>GSHMTITDVLKNTFNISPKPPRKFIAIDLGTTNSIAYIGGRGIIYNEASVMAYETGTKKLVALGEDARKLIGKTHDKIEIYTPLRNGAITDLRIAEEFIQHIGNRAKVQDVWKGSIVLIACPKSVTELERRAMVEMCKHLGADLVQVEEDTLMAALGAGANIFAPKGTFILDIGGGKTSAGIISAGGIVVSKSIKIAGNYIDEEILKYIRAKHTISIGVVTAEQIKKQIGSLYKGKETKKMVIFGRDVVTGMPKETEILDSEIRKLLISIFSSITQLVTDILESTPAELAGDAVMNGLLVSGGCAQISGLKEFLESYFQIPVKIAKNPQTAVIDGCIAYEKEIRDRLIEENKKNK[2x]

MreB is a bacterial protein belonging to the actin superfamily. This protein polymerizes into an antiparallel double-stranded filament that determines cell shape by maintaining cell wall synthesis. Here, we studied MreB3 and MreB5 in Spiroplasma eriocheiris (SpeMreB3 and SpeMreB5, respectively), a model organism for studying Spiroplasma swimming. SpeMreB3 adopts a canonical actin fold composed of four subdomains (IA, IB, IIA and IIB) and consists of the same secondary structure elements as CcMreB, Thermotoga maritima (Tm) MreB and SciMreB5, except for the C-terminal region.

The crystal structures of nucleotide-free (Nf) SpeMreB3 and its AMPPNP complex were determined at 1.90 and 1.75 Å resolution. The SpeMreB3-AMPPNP complex crystal includes two molecules (Mol-A and Mol-B) with an RMSD value estimated for Cα atoms of 0.891 Å. Thus, the SpeMreB3-AMPPNP complex crystal also contains antiparallel pairs of the protofilaments, although their arrangement differs from that of the Nf-SpeMreB3 crystal. The angle composed of centroids of subdomains IIB-IIA-IA (ω2) was more constant than ω1 among our crystal structures (ω2 = 88.9° for SpeMreB3-AMPPNP complex Mol-A, 90.3° for Mol-B and 91.2° for Nf-SpeMreB3), indicating that major structural changes upon nucleotide binding contribute to swing the subdomain IB. These conformational changes lead to the interaction between subdomains IIA and IB', which are absent in the Nf-SpeMreB3 protofilament. The interaction in SpeMreB3-AMPPNP complex Mol-A is mediated through a hydrogen-bonding network and is stabilized by an electrostatic interaction between D289 and K70’. The protofilament model of the SpeMreB3-AMPPNP complex fits well with the protofilament image in an antiparallel manner, suggesting that the protofilament structure in the double-stranded filament is the same as that in the crystal. In the SpeMreB3 structure, D147 and K174 are located at positions corresponding to E140 and T167 in CcMreB, respectively. However, D147 is far from the putative nucleophilic water molecule and K174 does not interact with water molecules. The residue corresponding to E169 is replaced by serine (S176) in SpeMreB3, which does not interact with K174.PARA-XYLENE | C8 H10 | 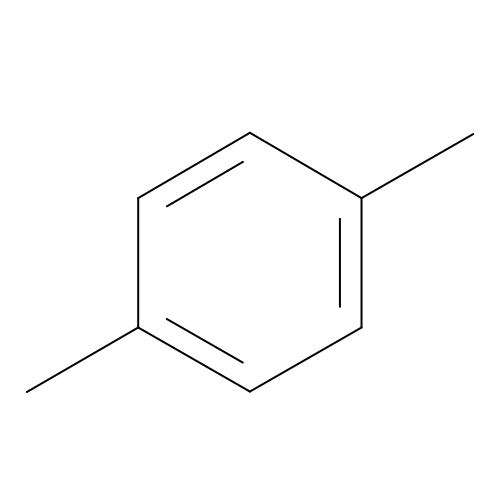URLKBWYHVLBVBO-UHFFFAOYSA-N>MGSSHHHHHHSSGLVPRGSHMSSSRSSSMDKTGWITHCFGRFLIDLPPDAVINAGYYLWGDRIEYLDDKPTELAARVDRLEQEWRTQRHKSKGNMFLRKIDFGNESVGLLSWSSEVASKTYLLDTYVTSKPTWHVYRWKGKVSVDREQHAVEISRALARNLRSRAPKEIPSEPGFCIDHAYIAGDSFQVERFGVGVTFPEHPGARFEFRSSTGAELNSLLERVDGFVQNMLSTFAGMETLRKGKHPVGSLPGEEYLVAGSDKGQRGYTFMWEVQGKEESLTEPNLTAGLAVLERSNENGKPPPPAFKSDKEALELWDTIVDSIRVRPTSSSPRGGNA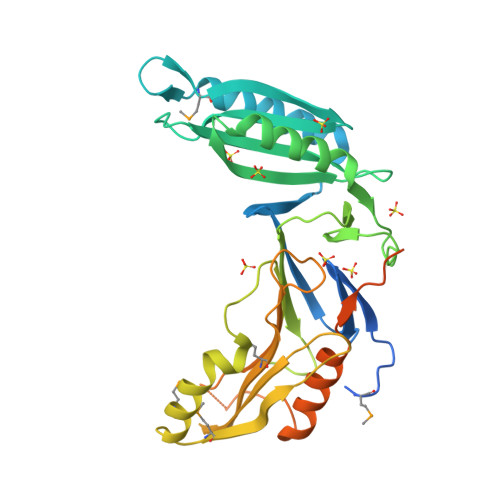GPSPAPKPATPGGQTLGDHYVYEEFLSSLKPKDSWLDDL[2x]>[2x]GPGSMSEKGRLFTSESVTEGHPDKICDAISDSVLDALLAQDPRSRVAVETLVTTGQVHVVGE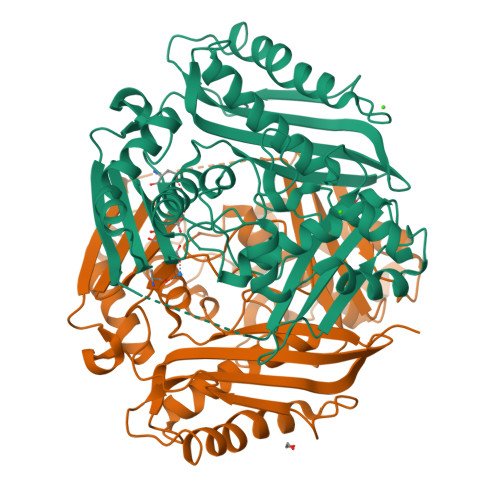VTTTAKEAFADITNTVRERILDIGYDSSDKGFDGASCGVNIGIGAQSPDIAQGVDTAHETRVEGAADPLDAQGAGDQGLMFGYAINDTPERMPLPIALAHRLSRRLTEVRKNGVLPYLRPDGKTQVTIEFEDDVPVRLDTVVISTQHAADIDLENTLTPDIREKVLNTVLNDLAHDTLDTSSTRLLVNPTGKFVVGGPMGDAGLTGRKIIVDTYGGWARHGGGAFSGKDPSKVDRSAAYAMRWVAKNIVAAGLAERVEVQVAYAIGKAAPVGLFIETFGTATVDPVKIEKIVPEVFDLRPGAIIRDLDLLRPIYAQTAAYGHFGRTDVELPWEQLNKVDDLKRAI> MENAHTKTVEEVLGHFGVNESTGLSLEQVKKLKERWGSNELPAEEGKTLLELVIEQFEDLLVRILLLAACISFVLAWFEEGEETITAFVEPFVILLILVANAIVGVWQERNAENAIEALKEYEPEMGKVYRQDRKSVQRIKAKDIVPGDIVEIAVGDKVPADIRLTSIKSTTLRVDQSILTGESVSVIKHTDPVPDPRAVNQDKKNMLFSGTNIAAGKAMGVVVATGVNTEIGKIRDEMVATEQERTPLQQKLDEFGEQLSKVISLICIAVWIINIGHFNDPVHGGSWIRGAIYYFKIAVALAVAAIPEGLPAVITTCLALGTRRMAKKN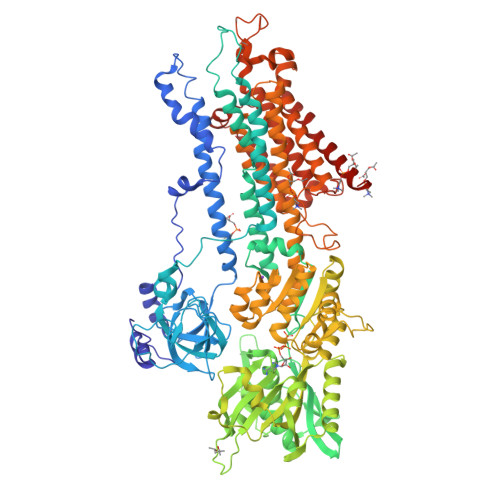AIVRSLPSVETLGCTSVICSDKTGTLTTNQMSVCRMFILDRVEGDTCSLNEFTITGSTYAPIGEVHKDDKPVNCHQYDGLVELATICALCNDSALDYNEAKGVYEKVGEATETALTCLVEKMNVFDTELKGLSKIERANACNSVIKQLMKKEFTLEFSRDRKSMSVYCTPNKPSRTSMSKMFVKGAPEGVIDRCTHIRVGSTKVPMTSGVKQKIMSVIREWGSGSDTLRCLALATHDNPLRREEMHLEDSANFIKYETNLTFVGCVGMLDPPRIEVASSVKLCRQAGIRVIMITGDNKGTAVAICRRIGIFGQDEDVTSKAFTGREFDELNPSAQRDACLNARCFARVEPSHKSKIVEFLQSFDEITAMTGDGVNDAPALKKAEIGIAMGSGTAVAKTASEMVLADDNFSTIVAAVEEGRAIYNNMKQFIRYLISSNVGEVVCIFLTAALGFPEALIPVQLLWVNLVTDGLPATALGFNPPDLDIMNKPPRNPKEPLISGWLFFRYLAIGCYVGAATVGAAAWWFIAADGGPRVSFYQLSHFLQCKEDNPDFEGVDCAIFESPYPMTMALSVLVTIEMCNALNSLSENQSLLRMPPWENIWLVGSICLSMSLHFLILYVEPLPLIFQITPLNVTQWLMVLKISLPVILMDETLKFVARNYLEPAILE> RDFNNLTKGLCTINSWHIYGKDNAVRIGEDSDVLVTREPYVSCDPDECRFYALSQGTTIRGKHSNGTIHDRSQYRALISWPLSSPPTVYNSRVECIGWSSTSCHDGKTRMSICISGPNNNASAVIWYNRRPVTEINTWARNILRTQESECVCHNGVCPVVFTDGSATGPAETRIYYFKEGKILKWEPLAGTAKHIEECSCYGERAEITCTCKDNWQGSNRPVIRIDPVAMTHTSQYICSPVLTDNPRP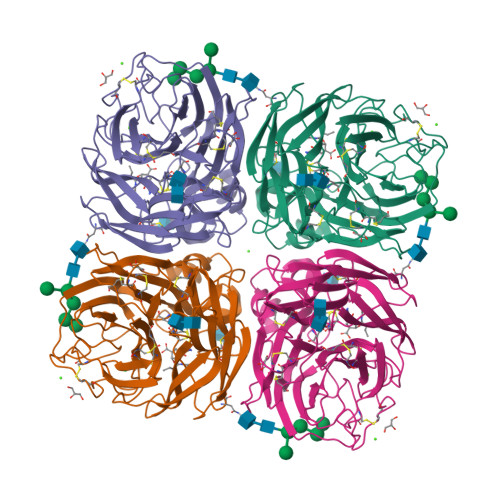NDPTVGKCNDPYPGNNNNGVKGFSYLDGVNTWLGRTISIASRSGYEMLKVPNALTDDKSKPTQGQTIVLNTDWSGYSGSFMDYWAEGECYRACFYVELIRGRPKEDKVWWTSNSIVSMCSSTEFLGQWDWPDGAKIEYFL> GVIKPDMKIKLKMEGNVNGHAFVIEGEGEGKPYDGTNTINLEVKEGAPLPFSYDILTTAFAYGNRAFTKYPDDIPNYFKQSFPEGYSWERTM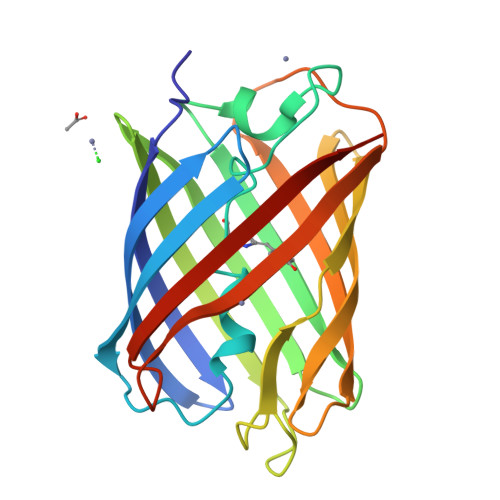TFEDKGIVKVKSDISMEEDSFIYEIHLKGENFPPNGPVMQKKTTGWDASTERMYVRDGVLKGDVKHKLLLEGGGHHRVDFKTIYRAKKAVKLPDYHFVDHRIEILNHDKDYNKVTVYESAVARNSTDGM> GAMADTQYILPNDIGVSSLDCREAFRLLSPTERLYAYHLSRAAWYGGLAVLLQTSPEAPYIYALLSRLFRAQDPDQLHQHALAEGLTEEEYQAFLVYAAGVYSNMGNYKSFGDTKFVPNLPKEKLERVILGSEAAQQHPEEVRGLWQTCGELMFSLEPRLRHLGLGKEGITTYFSGNCTMEDAKLAQDFLDSQNLSAYNTRLFKEVDGEGKPYYEVRLASVLGSEPSLDSEVTSKLKSYEFRGSPFQVTRGDYAPILQKVVEQLEKAKAYAANSHQGQMLAQYIESFTQGSIEAHKRGSRFWIQDKGPIVESYIGFIESYRDPFGSRGEFEGFVAVVNKAMSAKFERLVASAEQLLKELPWPPTFEKDKFLTPDFTSLDVLTFAGSGIPAGINIPNYDDLRQTEGFKNVSLGNVLAVAYATQREKLTFLEEDDKDLYILWKGPSFDVQVGLHELLGHGSGKLFVQDEKGAFNFDQETVINPETGEQIQSWYRSGETWDSKFSTIASSYEECRAESVGLYLCLHPQVLEIFGFEGADAEDVIYVNWLNMVRAGLLALEFYTPEAFNWRQAHMQARFVILRVLLEAGEGLVTITPTTGSDGRPDARVRLDRSKIRSVGKPALERFLRRLQVLKSTGDVAGGRALYEGYATVTDAPPECFLTLRDTVLLRKESRKLIVQPNTRLEGSDVQLLEYEASAAGLIRSFSERFPEDGPE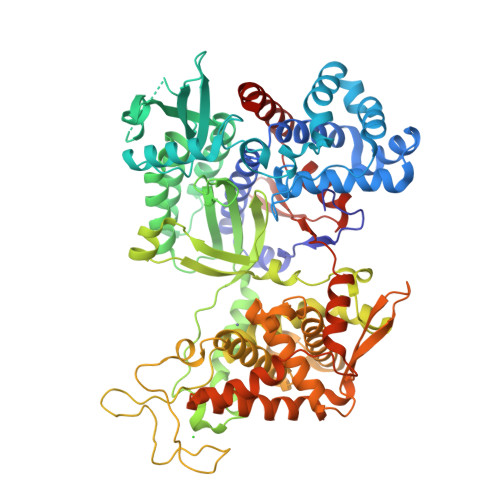LEEILTQLATADARFW>MNHKVHHHHHHIEGRHMTNTRSAVVLGGGMAGMLVSSMLARHVGSVTVIDRDAFPAGPDLRKGVPQARHAHILWSGGARIVEELLPGTTDRLLGAGAHRIGIPDGQVSYTAYGWQHRFPEAQFMIACSRALLDWTVREETLREERIALVEKTEVLALLGDAGRVTGVRVRDQESGEEREVPADLVVDTTGRGSPSKRLLAELGLPAPEEEFVDSGMVYATRLFRAPEAAATNFPLVSVHADHRAGRPGCNAVLMPIEDGRWIVTVSGTRGGEPPADDEGFARFARDGVRHPLVGELIAXAQPLTSVERSRSTVNRRLHYDRLATWPEGLVVLGDAVAAFNPVYGHGMSAAAHSVLALRSQLGQRAFQPGLARAAQRAIAVAVDDAWVLATSHDIGYPGCRTQTRDPRLTRHAGERQRVTDLVGLTATRNQVVNRAAVALNTLSAGMASMQDPAVMAAVRRGPEVPAPTEPPLRPDEVARLVSGAGVTA[2x]

In lasalocid A biosynthesis, a polyene polyketide intermediate is converted into a bisepoxide by the flavin‐dependent monooxygenase enzyme Lsd18. Remarkably, Lsd18 acts on two distinct C═C groups in the substrate molecule, forming two (R,R) epoxides. Like other members of the class A monooxygenase family, Lsd18 consists of a Rossmann‐like FAD binding domain and a β‐strand‐rich substrate binding domain. Our work has revealed that Lsd18 has an extra‐large substrate‐binding pocket that allows the polyene to adopt different conformations within the enzyme pocket.

To visualize how the substrate molecule binds in the active site, we determined the crystal structure of Lsd18‐FAD in complex with a diene substrate analogue, 1. The Lsd18‐FAD‐1 crystal structure was solved at 1.85 Å resolution with final R work and R free values of 0.16 and 0.20, respectively. Each Lsd18 contains one FAD, one substrate analogue, and one chloride ion. No electron density was observed for the oxazolidinone head group of 1, and therefore it was not modeled. The conformation of Lsd18 in the Lsd18‐FAD‐1 complex structure is nearly identical to that in the Lsd18‐FAD structure (RMSD = 0.13 Å). 1 is bound adjacent to the FAD isoalloxazine ring and makes contact with Lsd18 residues A70, I72, W74, Y218, H239, V252, and V342. Critically, the re face of the C19═C20 alkene of 1 is exposed to the active site cavity. In this configuration, transfer of an oxygen atom from the reactive C4a‐hydroperoxyflavin to the alkene is expected to produce an (R,R) epoxide, which is consistent with the structure of lasalocid A. We propose that the subpocket, formed by Y218, V252, and V342, and the nearby I72, determines the alkene binding orientation. In our crystal structure, the subpocket accommodates C19‐ethyl of 1, presumably generating binding free energy and promoting catalysis.methyl (3S)-3-hydroxydodecanoate | C13 H26 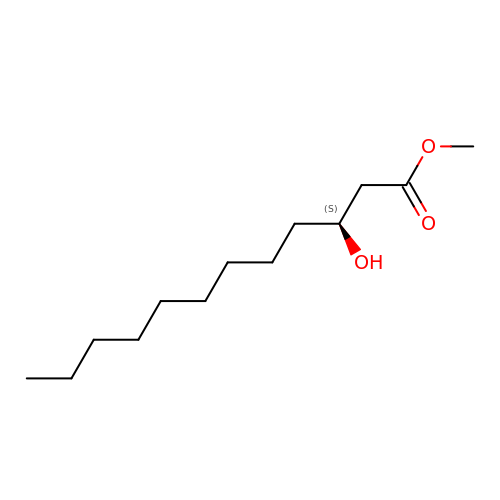O3 | OZXCINYANGIBDB-LBPRGKRZSA-N>[4x]MKLKAVHHVALIVSDYDKSYEFYVNQLGFEVIRENHRPKRHDYKLDLKCGDIELEIFGNKLTDSNYCAPPERISWPREACGL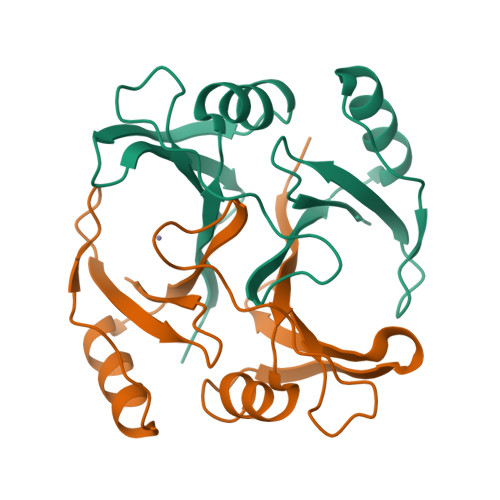RHLAFYVEDVEASRQELIALGIRVEEVRYDDYTGKKMAFFFDPDGLPLELHE1-methyl-5-(2'-methyl[1,1'-biphenyl]-4-yl)-1H-benzotriazole-7-carboxylic acid | C21 H17 N3 O2 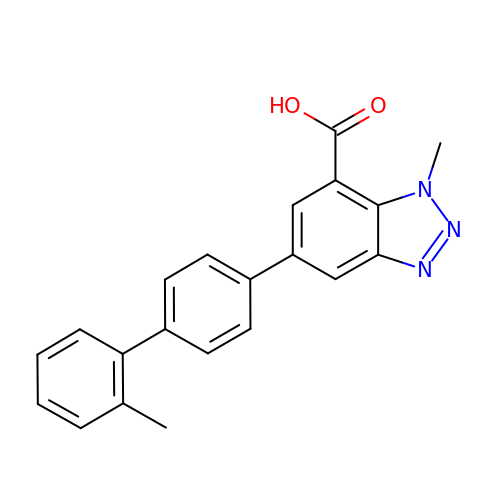| GSBZRCGZLMBSNY-UHFFFAOYSA-N> MASNSLEIEELARFAVDEHNKKENALLEFVRV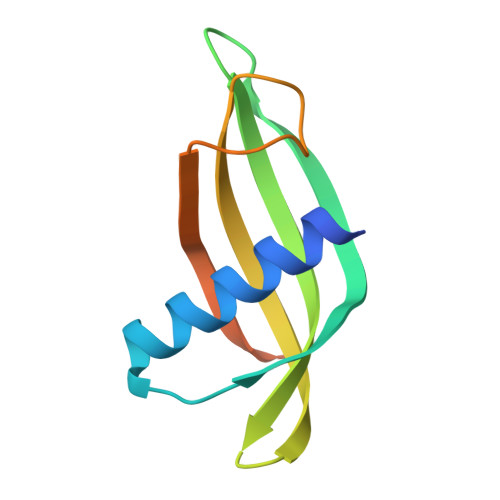VKAKEQLVGWVYEFQTMYYLTLEAKDGGKKKLYEAKVWVKSDHMPPSLPNFKELQEFKPVGDAAAAHHHHHHHH> KEEEDDDMK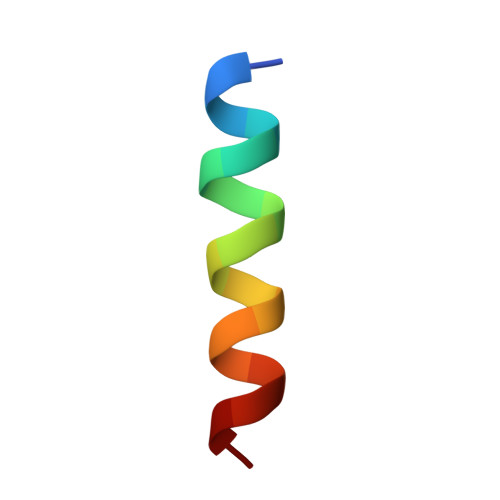ELENWAGSM> GPLGSTVDLDWKNLGFEYHKLPFRYISYYKDGKWDDGKLTEDATLHISESSPALHYGQEAFEGLKAYRTKDGSVQLFRPNMNAERLQRTADRLLMPQVPTDKFIDAAKQVVRANEEYVPPYGTGATLYLRPLLIGVGDVIGVHPADEYIFTIFAMPVGNYFKGGLAPTNFLIQDDYDRAAPHGTGAAKVGGNYAASLLPGKVAHERQFSDVIYLDPATHTKIEEVGSANFFGITKDNEFITPLSPSILPSVTKYSLLYLAEHRFGMKAIEG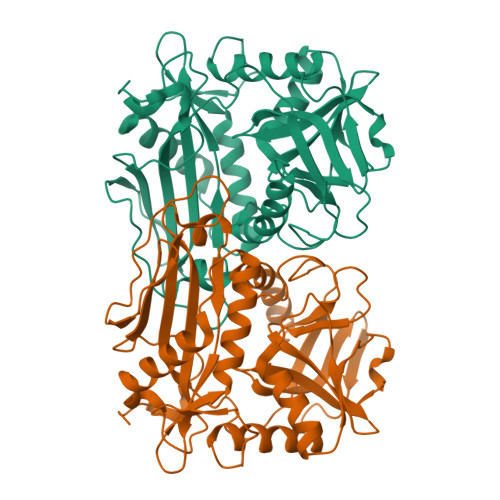DVCVDELDKFVEAGACGTAAVISPIGGVQHGDDFHVFYSETEVGPVTHKLYDELTGIQFGDVKAPEGWIYKVDD> MAAAALRRFWSRRRAEAGDAVVAKPGVWARLGSWARALLRDYAEACRDASAEARARPGRAAVYVGLLGGAAACFTLAPSEG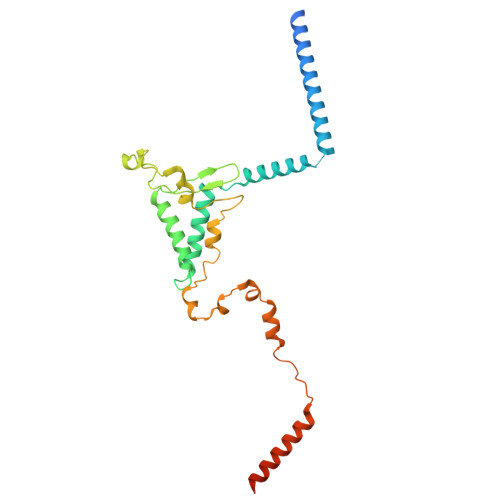AFEEALLEASGTLLLLAPATRNRESEAFVQRLLWLRGRGRLRYVNLGLCSLVYEAPFDAQASLYQARCRYLQPRWTDFPGRVLDVGFVGRWWVLGAWMRDCDINDDEFLHLPAHLRVVGPQQLHSETNERLFDEKYKPVVLTDDQVDQALWEEQVLQKEKKDRLALSQAHSLVQAEAPR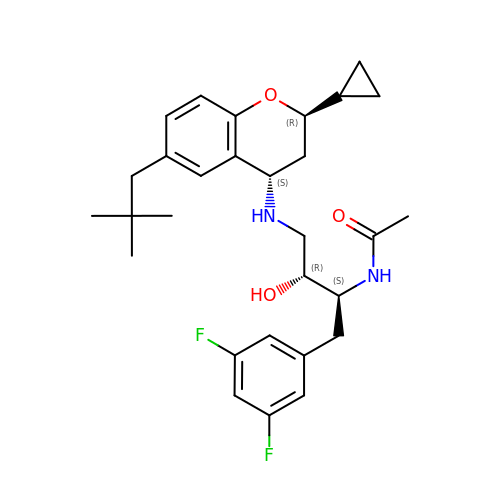N-[(2S,3R)-4-{[(2R,4S)-2-cyclopropyl-6-(2,2-dimethylpropyl)-3,4-dihydro-2H-chromen-4-yl]amino}-1-(3,5-difluorophenyl)-3-hydroxybutan-2-yl]acetamide | C29 H38 F2 N2 O3 | IBLLHMQPQAMFLM-WDTRASESSA-N To understand the molecular basis underlying the superbinding characteristics of the Legionella SH2 domains, we determined the structures of L. longbeachae LeSH and the L. pneumophila RavO SH2 domain in complex with tyrosine-phosphorylated peptides by X-ray crystallography. Compared to the Src SH2 domain, LeSH is missing two β-strands (βA and βF) but contains a 45-residue insert between the strand βE and the helix αB. This extra sequence in LeSH contains a structural motif called the pancreatic polypeptide (PP)-fold, comprising an amphipathic α-helix (named herein as αEF) packed against a polyproline segment via favorable hydrophobic contacts. Indeed, the SH2 and PP folds together form a clamp-like structure that grasp the pTyr residue.

We obtained crystal structures of LeSH in complex with three different pTyr ligands, including the phosphotyrosine itself, a 13-mer peptide derived from the pTyr381 site of DnaJ-A1, and another 13-mer peptide corresponding to the pTyr387 site in IL2Rβ. Apart from the pTyr residue, which assumed the same conformation in all three complexes, we were not able to detect the electron density for residues preceding the pTyr in the DnaJ-A1 peptide or any residues flanking the pTyr in the IL2Rβ peptide despite the high resolution (1.6–1.7 Å) of the complex structures obtained. Furthermore, deletion of either the N- or the C-terminal region from the DnaJ-A1 peptide (DnaJ-A1-pTyr381 ∆N or ∆C) had no apparent impact on binding to LeSH or other Legionella SH2 domains, suggesting that neither the N- or C-terminal residues contribute to binding. In accordance with this observation, no electron density was detected for residues flanking the pTyr in the DnaJ-A1 peptide in complex with LeSH. However, LeSH lacks a pocket for the accommodation of a C-terminal residue to the pTyr. Consequently, LeSH features a rather flat surface in the equivalent P + 3/P + 4-binding area. This explains the results from the peptide array screening showing minimal sequence selectivity by LeSH. However, the R46K mutant of LeSH bound the DnaJ-A1 and IL2βR peptides that contain multiple Asp/Glu residues markedly better than to the remaining peptides that contain fewer acidic residues. This indicates that charge–charge interaction plays a pivotal role in the LeSH-peptide ligand interaction.

> GAMEAMQKNELNSKIPIIFGLINSYQIHNLLEQHNAKTKESKAVFLIRDSSTYPGLLTISYYCQEQDIVKHIRFGLTDKGWKTAPKPPHEPLKSDSPEIKEKYTLDKIKFERKMKQFINTAKKLFEQHIRAESFKTLIMELKIHEFNLEGLIKPTRSQASQEKHFTDYV;> HYNGEAYEDDEHH>[2x]GPLGSSTEEEEERLEREHFWKIINAFRYYGTSMHERVNRTERQFRSLPANQQKLLPQFLLHLDKIRKCIDHNQEILLTIV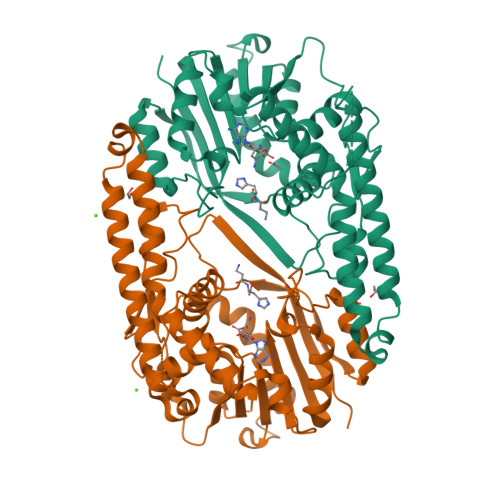NDCIHMFENKEYGEDGNGKIMPASTFDMDKLKSTLKQFVRDWSETGKAERDACYQPIIKEILKNFPKERWDPSKVNILVPGAGLGRLAWEIAMLGYACQGNEWSFFMLFSSNFVLNRCSEINKYKLYPWIHQFSNNRRSADQIRPIFFPDVDPHSLPPGSNFSMTAGDFQEIYSECNTWDCIATCFFIDTAHNVIDYIDTIWKILKPGGIWINLGPLLYHFENLANELSIELSYEDIKNVVLQYGFKVEVEKESVLSTYTVNDLSMMKYYYECVLFVVRKPQ> YAIAGNGVRVTYDADGQTITLYRTEGSGLIQMSKPSPLGGPVVGGQEVQDFSHISCDVEQSTSGVMGSGQRMTITSQSMSTGLIRTYVLETSDIEEGVVYTATSYEAGASDVEVSWFIGSVYELYGAEDRIWSYNGGGEGPMHYYDTLQKIDLTDSGKFSRENKQDDTAASIPVSDIYIADGGITVGDASATRREVHTPVQETSDSAQVSIGWPGKVIAAGSVIEIGESFAVVHPGDYYNG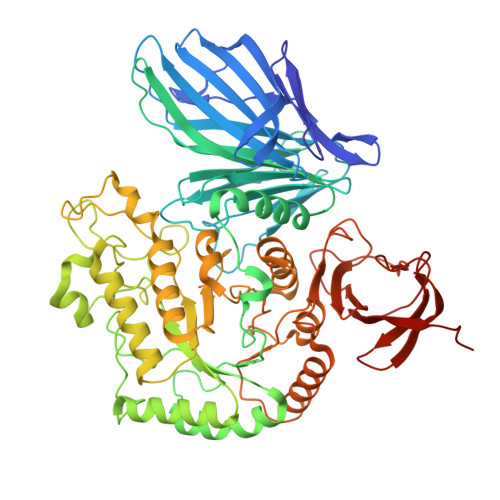LRGYKNAMDHLGVIMPAPGDIPDSSYDLRWESWGWGFNWTIDLIIGKLDELQAAGVKQITLDDGWYTNAGDWALNPEKFPNGASDALRLTDAIHEHGMTALLWWRPCDGGIDSILYQQHPEYFVMDADGRPARLPTPGGGTNPSLGYALCPMADGAIASQVDFVNRAMNDWGFDGFKGDYVWSMPECYNPAHNHASPEESTEKQSEIYRVSYEAMVANDPNVFNLLCNCGTPQDYYSLPYMTQIATADPTSVDQTRRRVKAYKALMGDYFPVTADHNNIWYLSAVGTGSVLIEKRDLSGTAKEEYEKWLGIADTVQLQKGRFIGDLYSYGFDPYETYVVEKDGVMYYAFYKDGSKYSPTGYPDIELKGLDPNKMYRIVDYVNDRVVATNLMGDNAVFNTRFSDYLLVKAVEISEPDP>[2x]VEYRNWSKPQCQITGFAPFSKDNSIRLSAGGDIWVTREPYVSCDPGKCYQFALGQGTTLDNKHSNDTVHDRIPHRTLLMNELGVPFHLGTRQVCI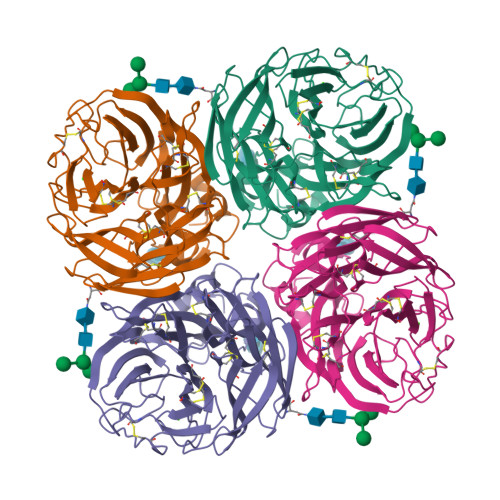AWSSSSCHDGKAWLHVCITGDDKNATASFIYDGRLVDSIGSWSQNILRTQESECVCINGTCTVVMTDGSASGRADTRILFIEEGKIVHISPLSGSAQHIEECSCYPRYPGVRCICRDNWKGSNRPVVDINMEDYSIDSSYVCSGLVGDTPRNDDSSSNSNCRNPNNERGTQGVKGWAFDNGNDLWMGRTISKESRSGYETFKVIGGWSTPNSKSQVNRQVIVDNNNWSGYSGIFSVEGKSCINRCFYVELIRGRPQETRVWWTSNSIVVFCGTSGTYGTGSWPDGANINFMPI>RLPRETDEEPEEPGRRGSFVEMVDNLRGKSGQGYYVEMTVGSPPQTLNILVDTGSSNFAVGAAPHPFLHRYYQRQLSSTYRDLRKGVYVPYTQGKWEGELGTDLVSIPHGPNVTVRANIAAITESDKFFINGSNWEGILGLAYAEIARPDDSLEPFFDSLVKQTHVPNLFSLQLCGAGFPLNQSEVLASVGGSMIIGGIDHSLYTGSLWYTPIRREWYYEVIIVRVEINGQDLKMDCKEYNYDKSIVDSGTTNLRLPKKVFEAAVKSIKAASSTEKFPDGFWLGEQLVCWQAGTTP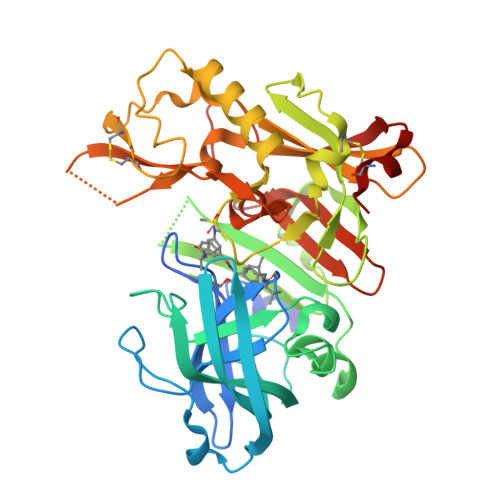WNIFPVISLYLMGEVTNQSFRITILPQQYLRPVEDVATSQDDCYKFAISQSSTGTVMGAVIMEGFYVVFDRARKRIGFAVSACHVHDEFRTAAVEGPFVTLDMEDCGYN[3x]>MEEAYLALGKKILEEGHFKEDRTGTGTYSLFGYQMRFDLAKGFPLLTTKRVPFGLIKSELLWFLKGDTNIRYLLERNNHIWDEWAFERYVKSADYQGPDMTDFGHRVLQDPAFAEQYKEEHQKFCDAILNDAEFAEKYGELGNIYGAQWRHWETKDGSFIDQLANVIEMIKTNPDSRRLIVSAWNPEDVPSMALPPCHTMFQFYVNEGKLSCQLYQRSADVFLGVPFNIASYALLTHLIAHETGLEVGEFVHTLGDAHLYQNHVEQMQEQLSREVRSFPTLVLNPDKASVFDFDMEDIKVEGYDPHPTIKA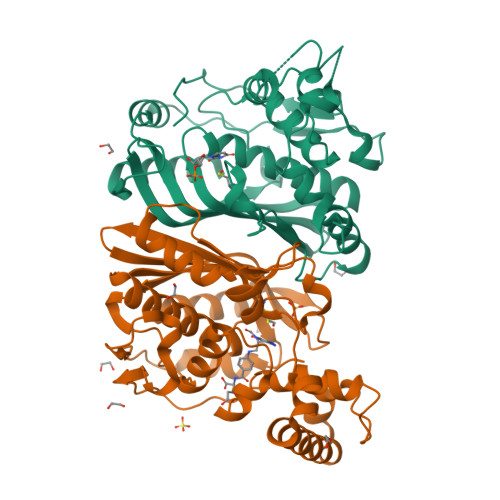PIAV[4x]>[5x]GGAACCGGUGCGCAUAACCACCUCA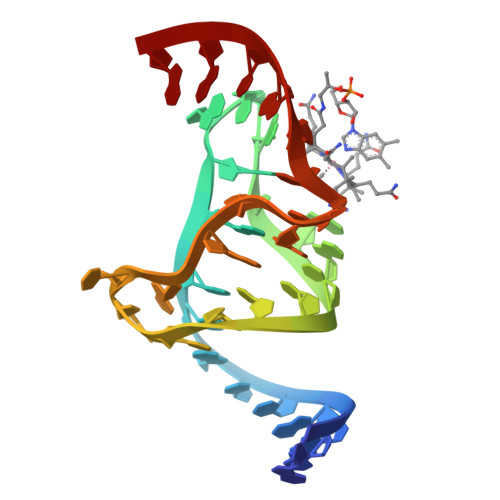GUGCGAGCAA> ASMTGGQQMGRGSASLPACPEESPLLVGPMLIEFNMPVDLELV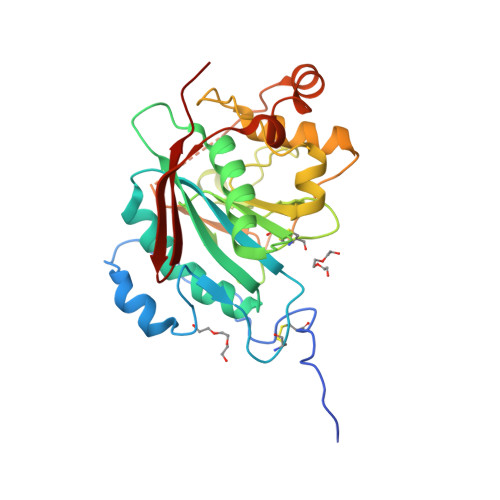AKQNPNVKMGGRYAPRDCVSPHKVAIIIPFRNRQEHLKYWLYYLHPVLQRQQLDYGIYVINQAGDTIFNRAKLLNVGFQEALKDYDYTCFVFSDVDLIPMNDHNAYRCFSQPRHISVAMDKFGFSLPYVQYFGGVSALSKQQFLTINGFPNNYWGWGGEDDDIFNRLVFRGMSISRPNAVVGTTRHIRHSRDKKNEPNPQRFDRIAHTKETMLSDGLNSLTYQVLDVQRYPLYTQITVDIGTPS>MNISSAQFIPGVHTVEEIEAEIHKNLHISKSCSYQKVPNSHKEFTKFCYEVYNEIKISDKEFKEKRAALDTLRLCLKRISPDAELVAFGSLESGLALKNSDMDLCVLMDSRVQSDTIALQFYEELIAEGFEGKFLQRARIPIIKLTSDTKNGFGASFQCDIGFNNRLAIHNTLLLSSYTKLDARLKPMVLLVKHWAKRKQINSPYFGTLSSYGYVLMVLYYLIHVIKPPVFPNLLLSPLKQEKIVDGFDVGFDDKLEDIPPSQNYSSL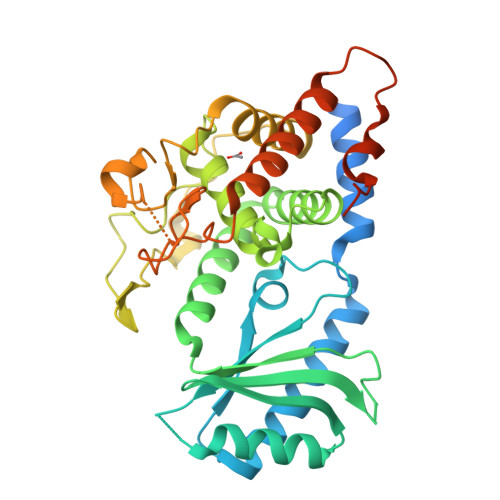GSLLHGFFRFYAYKFEPREKVVTFRRPDGYLTKQEKGWTSATEHTGSADQIIKDRYILAIEDPFEISHNVGRTVSSSGLYRIRGEFMAASRLLNSRSYPIPYDSLFEEAPIPPRRQKKTDEQSNKKLLNETDGDNSE[4x]>MESLKTDTEMPYPEVIVDVGRVIFGEENRKKMTNSCLKRSENSRIIRAICALLNSGGGVIKAEIDDKTYSYQCHGLGQDLETSFQKLLPSGSQKYLDYMQQGHNLLIFVKSWSPDVFSLPLRICSLRSNLYRRDVTSAINLSASSALELLREKGFRAQRGRPRVKKLHPQQVLNRCIQEEEDMRILASEFFKKDKLMYKEKLNFTESTHVAFKRFTTKKVIPRIKEMLPHYVSAFANTQGGYVLIGVDDKSKEVVGCKWEKVNPDLLKKEIENCIEKLPTFHFCCEKPKVNFTTKILNVYQKDVLDGYVCVIQVEPFCCVVFAEAPDSWIMKDNSVTRLTAEQWVVMMLDTQSAPPSLVTDYNSSLISSASSARKSPGYPIKVHKFKEALQRHLFPVTQEEVQFKPESLCKKLFSDHKELEGLMKTLIHPCSQGIVIFSRSWAGDVGFRKEQNVLCDALLIAVNSPVVLYTILIDPNWPGGLEYARNTAHQLKQKLQTVGGYTGKVCIIPRLIHLSSTQSRPGEIPLRYPRSYRLADEEEMEDLLQALVVVSLSSRSLLSDQMGCEFFNLLIMEQSQLLSESLQKTRELFIYCFPGVRKTALAIKIMEKIKDLFHCKPKEILYVCESDSLKDFVTQQTTCQAVTRKTFMQGEFLKIKHIVMDETENFCSKYGNWYMKAKNITHPKAKGTGSENLHHGILWLFLDPFQIHHADVNGLPPPSAQFPRKTITSGIHCALEIAKVMKEEMKRIKENPPSNMSPDTLALFSETAYEEATSAQALPGVCETKTNLTTEQIANYVARKCHSLFQSGYLPKDIAILCRRGEDRGRYRLALLKAMELIETHRPSEVVFSPATGVWGSHIVLDSIQQFSGLERTVVFGLSPECDQSEEFHKLCFASRAIKHLYLLYEKRAAY[2x]

SLFN14 is another important member of the SLFN family (group III proteins containing RNase, SWAVDL, and helicase domains) that shares domain organization with SLFN11 and SLFN13. Herein, we carried out a systematic characterization of the enzymatic activities of human SLFN14, revealing that SLFN14 has RNase activity that cleaves RNAs containing double‐strand regions. By determining cryogenic electron microscopy (cryo‐EM) structures of SLFN14 apoenzyme and SLNF14 bound to a short hairpin RNA, we demonstrate that SLFN14 assembles into a ring‐like homodimer, and that an RNA‐binding groove formed by the two SLFN14‐NTD domains can accommodate a short hairpin RNA of ∼12 bp. The SLFN14 RNase domain is followed by a linker domain (366‐571 aa) and a superfamily I helicase domain (572‐912 aa).

To reveal the structural details underpinning the function of SLFN14, we determined the cryo‐EM structures of the full‐length human SLFN14 apoenzyme. Because wild‐type (WT) SLFN14 protein was not suitable for single‐particle analysis, primarily because it strongly aggregated on the cryo‐EM grid, we introduced four mutations, i.e., E211A, C365S, C775S, and C808S into SLFN14 (denoted SLFN14mut) to circumvent this problem. SLFN14mut was more stable and soluble, which allowed us to perform 3D reconstruction of the sample using ≈0.96 million particles, yielding an interpretable EM density map with an overall resolution of 2.84 Å that was suitable for model building. The cryo‐EM structure of apo SLFN14mut features a dimer with an overall fold similar to that of the SLFN11 dimer. Specifically, two intertwined SLFN14 monomers are organized with C2 symmetry, forming a ring‐like architecture. This ring‐like architecture of SLFN14 is composed of two copies of SWAGDV motif and helicase domain forming the body of the ring and two copies of N‐terminal RNase domains organized head‐to‐tail, forming a central RNA binding groove on top of the ring. SLFN14 harbors a zinc‐finger module located at the C‐lobe of the RNase domain, where a zinc ion is coordinated by residues C318, C319, H282, and C284. Using software PISA (Proteins, Interfaces, Structures and Assemblies), we calculated the dimer interfacial area for SLFN14 as 2807Å2 (ΔG = −17.9 kcal mol−1), which is larger than that of SLFN11 dimer interfacial area, 1848Å2 (ΔG = −1.1 kcal mol−1). Additionally, the ID‐helix in SLFN14 blocks access to the ATP‐binding pocket, as observed previously for the autoinhibited ATPase conformation observed in SLFN11. By contrast, in the SLFN14 apoenzyme structure, K213, R214, and F215 on Loop 211–220 are shifted away from the active site, suggesting the SLFN14 apoenzyme structure may represent the RNase inactive state of the enzyme.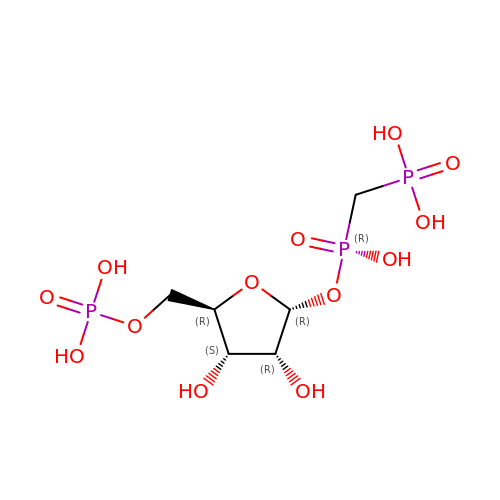1-O-[(R)-hydroxy(phosphonomethyl)phosphoryl]-5-O-phosphono-alpha-D-ribofuranose | C6 H15 O13 P3 | JFMKBQDEISBIPL-KVTDHHQDSA-N> DQAGKSPAGVRYHGGDEIILQGFHWNVVREAPNDWYNILRQQASTIAADGFSAIWMPVPWRDFSSWTDGGKSGGGEGYFWHDFNKNGRYGSDAQLRQAAGALGGAGVKVLYDVVPNHMNRGYPDKEINLPAGQGFWRNDCADPGNYPNDCDDGDRFIGGESDLNTGHPQIYGMFRDELANLRSGYGAGGFRFDFVRGYAPERVDSWMSDSADSSFCVGELWKGPSEYPSWDWRNTASWQQIIKDWSDRAKCPVFDFALKERMQN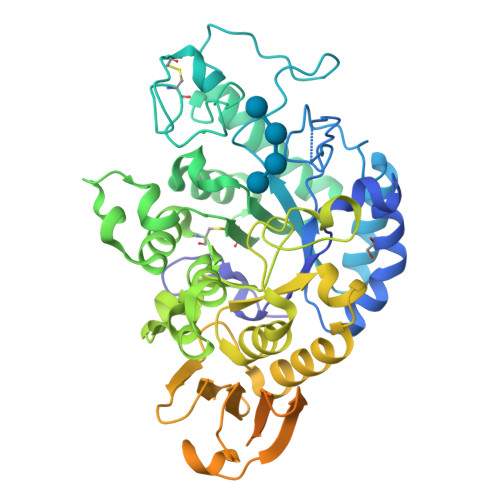GSVADWKHGLNGNPDPRWREVAVTFVDNHDTGYSPGQNGGQHHWALQDGLIRQAYAYILTSPGTPVVYWSHMYDWGYGDFIRQLIQVRRTAGVRADSAISFHSGYSGLVATVSGSQQTLVVALNSDLANPGQVASGSFSEAVNASNGQVRVWRSGSGDGGGNDGGEGGLVNVNFRCDNGVTQMGDSVYAVGNVSQLGNWSPASAVRLTDTSSYPTWKGSIALPDGQNVEWKCLIRNEADATLVRQWQSGGNNQVQAAAGASTSGSFHHHHHH>MARFNAAFTRIKIMFSRIRGLISCQSNTQTIAPTLSPPSSGHVSFAGIDYPLLPLNHQTPLVFQWFERNPDRFGQNEIPIINTQKNPYLNNIINAAIIEKERIIGIFVDGDFSKGQRKALGKLEQNYRNIKVIYNSDLNYSMYDKKLTTIYLENITKLEAQSASERDEVLLNGVKKSLEDVLKNNPEETLISSHNKDKGHLWFDFYRNLFLLKGSDAFLEAGKPGCHHLQPGGGCIYLDADMLLTDKLGTLYLPDGIAIHVSRKDNHVSLENGIIAVNRSEHPALIKGLEIMHSKPYGDPYNDWLSKGLRHYFDGSHIQDYDAFCDF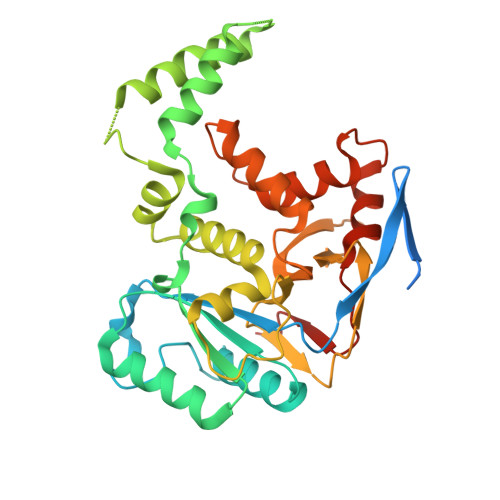IEFKHENIIMNTSSLTASSWR[2x]(2~{R},3~{S},4~{S},5~{R},6~{R})-6-(hydroxymethyl)-4-[(2~{S},3~{R},4~{S},5~{S},6~{R})-6-(hydroxymethyl)-3,4,5-tris(oxidanyl)oxan-2-yl]sulfanyl-oxane-2,3,5-triol 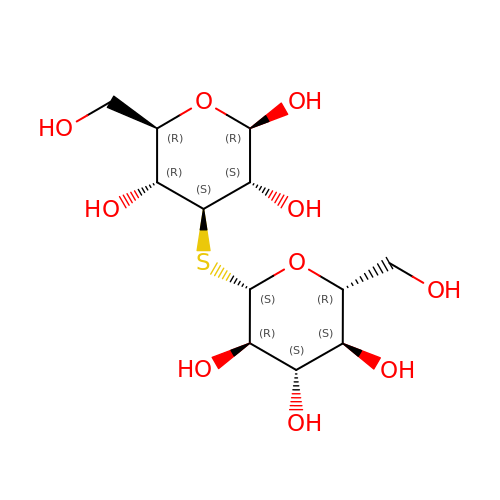| C12 H22 O10 S | XRTVCRDMGYFFNB-CSOAUFAESA-N>[4x]MGHHHHHHVEKVATNVNLKDQFWKRYIDVVRHEVIPYQWEALNDRIPDAEPSHAIENFRIAAGESDGEFYGMVFQDSDVAKWLEAVAYLLETKRDPELEKLADDVIELLGRAQQPDGYLNTYYTIKEPGKRWMNLRDNHELYCAGHLIEAAVAYFRATGKRRFLDIMCKYA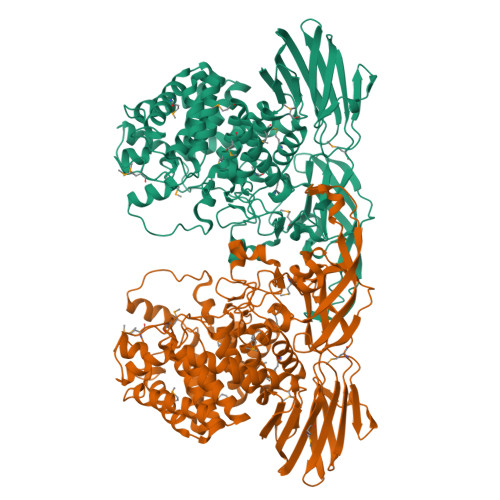DYIGTVFGRGEGQIPGYDGHQEIELALLKLYEVTGNENYLKLSQYFIDQRGQQPYYFDQEKEARGETEPFWYDGGYRYHQAHIPVREQKQAVGHAVRALYMYTAMAGLAAKMGDESLKQACQTLWENVTKRQMYITGGVGSSAFGESFTFDFDLPNDTAYAETCASIALVFWTRRMLELEMDGKYADVMERALYNGTISGMDLDGKKFFYVNPLEVWPKACERHDKRHVKPVRQKWFSCACCPPNLARLIASIGHYIYLQTSDALFVHLYVGSDIQTEIDGRSVKIMQETNYPWDGTVRLTVSPESAGEFTLGLRIPGWCRGAEVTINGEKVDIVPLIKKGYAYIRRVWQQGDEVKLYFPMPVERIKAHPQVRANAGKVALQRGPIVYCLEEVDNGPNLANLFLPRDAKLEAHFEPDLLEGVVVITGIAERVDESAWNDELYRPIEPRTYKVPFRAIPYYAWCNRGEGEMVVWVNEK ACTINONIN | C19 H35 N3 O5 | 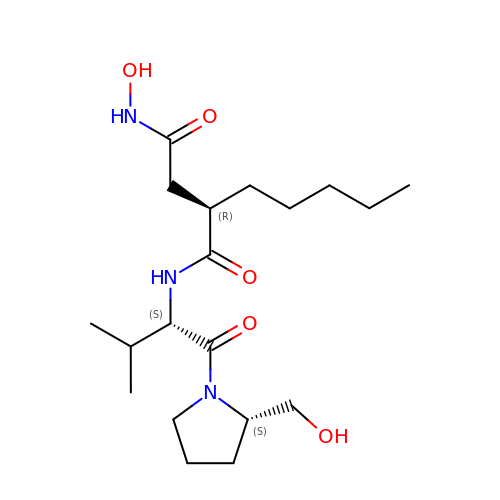XJLATMLVMSFZBN-VYDXJSESSA-N>[3x]MSDGSRHSMHQVLETVYGEVPATPAFKRIRHNSTTLATAINTLTSEELRPDRNSMGIRHGTRQVGGEIVSELSFESLDDTLEALMCGTWNADALVNGVTRRSFSILRQFNDLTSASLPNFVYVGCEYNTMTLSITTEAIVMATFGIVGMNQLEPSSTVPTGATFVEAPTTEPMDSFTGHVKEGLADIAVA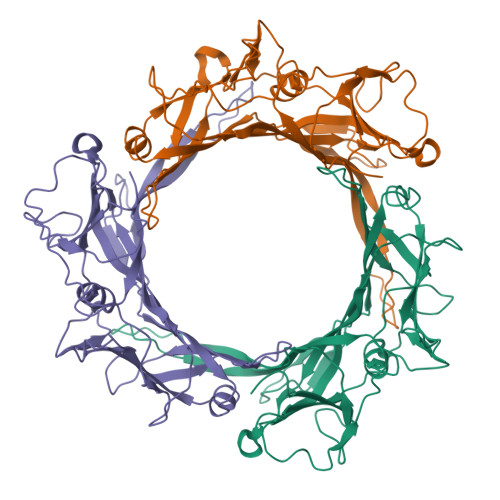TELELQIENGIAPRYVIGSKKSIKQSIGRFKVSGTLTAYFEDATLVGKFLREEASSLEFVVTDGLAGNSYKFELPKIKYTGGQPDVGGEGPITLSMPFVAEYDPTILGTLKITRIGA> SVKNETVKLSVGTVSGNPGDTVKVPVTISQVSTPVGLICMDISYDASKFTVKDVLPNTDLVKDTDNYSFIVNTSTPGKISITFTDPTLANYPISVDGILAYLDFIINSNATAGDSALTVDPATLIVADENDKDIKDAASNGKITVTGSAP;> SNTILGDLNDDGVVNGRDIVMMRQYLAGKTVSG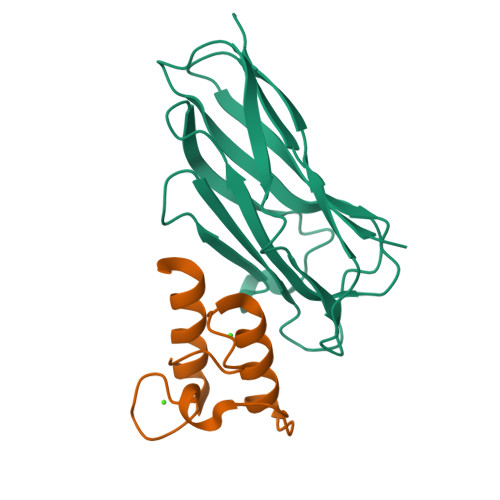IDKNALDINGDGAVNGDDLMELIKKVSNN Glycolyl-CoA carboxylase (GCC) is a new-to-nature enzyme that catalyzes the key reaction in the tartronyl-CoA (TaCo) pathway, a synthetic photorespiration bypass that was recently designed to improve photosynthetic CO2 fixation. GCC was created from propionyl-CoA carboxylase (PCC) through five mutations. The enzyme forms an α6β6 dodecameric complex, where the β-subunits arrange in a central core of two trimeric layers, while the α-subunits sit on top of the core and face outward. The biotin cofactor that is essential to catalysis is covalently linked to a lysine residue in the BCCP domain of the α-subunit and acts as a flexible arm that transfers the carboxyl group derived from HCO3– between the active sites of the α- and β-subunits.

Among the tested candidates, variant G20R stood out with a specific activity for glycolyl-CoA carboxylation of 2.6 ± 0.4 μmol min–1 mg–1 at a concentration of 0.5 mM glycolyl-CoA, which corresponded to a 2.8-fold improvement of the carboxylation rate compared to that of GCC M5. While the apparent KM value for glycolyl-CoA slightly increased, the Vmax was 1.8-fold higher than that of GCC M5 and thus the G20R variant with a kcat of 9.8 ± 0.2 represents a very promising candidate for GCC-based applications. In this variant, the substitution of Gly by Arg on a surface loop of the β-core strongly increased the carboxylation rate, whereas the ATP per carboxylation ratio changed only marginally. To identify structural changes that might be responsible for the catalytic improvements of the G20R or L100N variants, we solved their cryo-EM structures at 2.05 and 2.31 Å, respectively. The G20R substitution is located ∼8 Å away from the 3′-phosphate of coenzyme A and has no obvious interactions with other residues or the substrate. The lack of defined contact points in the cryo-EM structure is reflected in only weak electron density observed for the side chain of Arg20, indicating a high degree of side chain flexibility. Arg20 is positioned in a flexible loop, where it is preceded by two glycine residues, which add to its increased flexibility. Based on G20R’s position on the top rim of the β6 core of GCC, we suspected that it might help stabilize the interaction with the α-subunit and indirectly also facilitate CoA positioning. Indeed, in mass photometry (MP) measurements, the G20R variant formed more higher mass complexes relative to GCC M5, indicating a more stable complex formation. Thus, the higher fraction of α-subunits bound to the β6 core likely explains the higher in vitro activity of the G20R mutant.

>[6x]MKDILEKLEERRAQARLGGREKRLEAQHKRGKLTARERIELLLDHGSFEEFDMFVQHRSTDFGMEKQKIPGDGVVTGWGTVNGRTVFLFSKDFTVFGGSSSEAHAAKIVKVQDMALKMRAPIIGIFDAGGARIQEGVAALGGHGEVFRRNVAASGVIPQISVIMGPCAGGDVYSPAMTDFIFMVRDTSYMFVTGPDVVKTVTNEVVTAEELGGAKVHTSKSSIADGSFENDVEAILQIRRLLDFLPANNIEGVPEIESFDDVNRLDKSLDTLIPDNPNKPYDMGELIRRVVDEGDFFEIQAAYARNIITGFGRVEGRTVGFVANQPLVLAGVLDSDASRKAARFVRFCNAFSIPIVTFVDVPGFLPGTAQEYGGLIKHGAKLLFAYSQATVPLVTIITRKAFGGAYIVMASKHVGADLNYAWPTAQIAVMGAKGAVEIIFRAEIGDADKVAERTKEYEDRFLSPFVAAERGYIDEVIMPHSTRKRIARALGMLRTKEMEQPRKKHDNIPL;>MFDKILIANRGEIACRIIKTAQKMGIKTVAVYSDADRDAVHVAMADEAVHIGPAPAAQSYLLIEKIIDACKQTGAQAVHPGYGFLSERESFPKALAEAGIVFIGPNPGAIAAMGDKIESKKAAAAAEVSTVPGFLGVIESPEHAVTIADEIGYPVMIKASAGGGGKGMRIAESADEVAEGFARAKSEASSSFGDDRVFVEKFITDPRHIEIQVIGDKHGNVIYLGERECSIQRRNQKVIEEAPSPLLDEETRRKMGEQAVALAKAVNYDSAGTVEFVAGQDKSFYFLEMNTRLQVEHPVTEMITGLDLVELMIRVAAGEKLPLSQDQVKLDGWAVESRVYAEDPTRNFLPSIGRLTTYQPPEEGPLGGAIVRNDTGVEEGGEIAIHYDPMIAKLVTWAPTRLEAIEAQATALDAFAIEGIRHNIPFLATLMAHPRWRDGRLSTGFIKEEFPEGFIAPEPEGPVAHRLAAVAAAIDHKLNIRKRGISGQMRDPSLLTFQRERVVVLSGQRFNVTVDPDGDDLLVTFDDGTTAPVRSAWRPGAPVWSGTVGDQSVAIQVRPLLNGVFLQHAGAAAEARVFTRREAELADLMPVKENAGSGKQLLCPMPGLVKQIMVSEGQEVKNGEPLAIVEAMKMENVLRAERDGTISKIAAKEGDSLAVDAVILEFA[6x]> 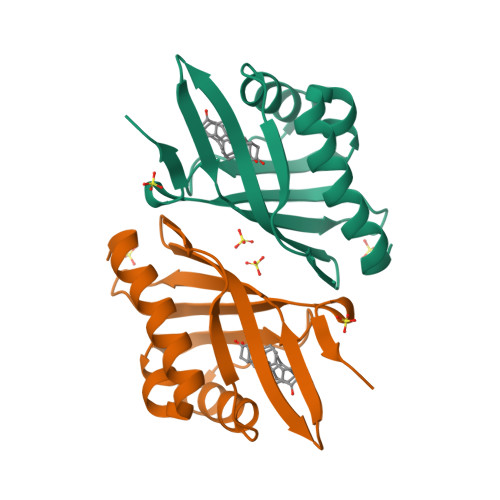MNTPEHMTAVVQRYVAALNAGDLDGIVALFADDATVENGVGSEPRSGTAAIREFYANSLKLPLAVELTQEVRAVANEAAFAFTVSFEYQGRKTVVAPINHFRFNGAGKVVSMRALFGEKNIHAGA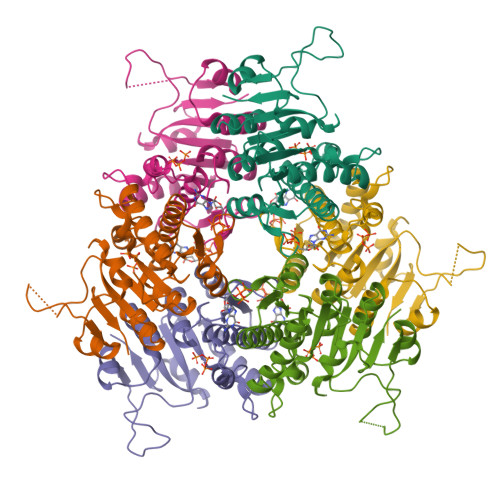>MATNAKPVYKRILLKLSGEALQGTEGFGIDASILDRMAQEIKELVELGIQVGVVIGGGNLFRGAGLAKAGMNRVVGDHMGMLATVMNGLAMRDALHRAYVNARLMSAIPLNGVCDSYSWAEAISLLRNNRVVILSAGTGNPFFTTDSAACLRGIEIEANVVLKATKVDGVFTADPAKDPTATMYEQLTYSEVLEKELKVMDLAAFTLARDHKLPIRVFNMNKPGALRRVVMGEKEGTLITE[6x]>PHMQPFDSGHDDLVHDVVYDFYGRHVATCSSDQHIKVFKLDKDTSNWELSDSWRAHDSSIVAIDWASPEYGRIIASASYDKTVKLWEEDPDQEECSGRRWNKLCTLNDSKGSLYSVKFAPAHLGLKLACLGNDGILRLYDALEPSDLRSWTLTSEMKVLSIPPANHLQSDFCLSWCPSRFSPEKLAVSALEQAIIYQRGKDGKLHVAAKLPGHKSLIRSISWAPSIGRWYQLIATGCKDGRIRIFKITEKLSPLASEESLTNSNMFDNSADVDMDAQGRSDSNTEEKAELQSNLQVELLSEHDDHNGEVWSVSWNLTGTILSSAGDDGKVRLWKATYSNEFKCMSVITAQQ[4x];>MTIDDSNRLLMDVDQFDFLDDGTAQLSNNKTDEEEQLYKRDPVSGAILVPMTVNDQPIEKNGDKMPLKFKLGPLSYQNMAFITAKDKYKLYPVRIPRLDTSKEFSAYVSGLFEIYRDLGDDRVFNVPTIGVVNSNFAKEHNATVNLAMEAILNELEVFIGRVKDQDGRVNRFYELEESLTVLNCLRTMYFILDGQDVEENRSEFIESLLNWINRSDGEPDEEYIEQVFSVKDSTAGKKVFETQYFWKLLNQLVLRGLLSQAIGCIERSDLLPYLSDTCAVSFDAVSDSIELLKQYPKDSSSTFREWKNLVLKLSQAFGSSATDISGELRDYIEDFLLVIGGNQRKILQYSRTWYESFCGFLLYYIPSLELSAEYLQMSLEANVVDITNDWEQPCVDIISGKIHSILPVMESLDSCTAAFTAMICEAKGLIENIFEGEKNSDDYSNEDNEMLEDLFSYRNGMASYMLNSFAFELCSLGDKELWPVAIGL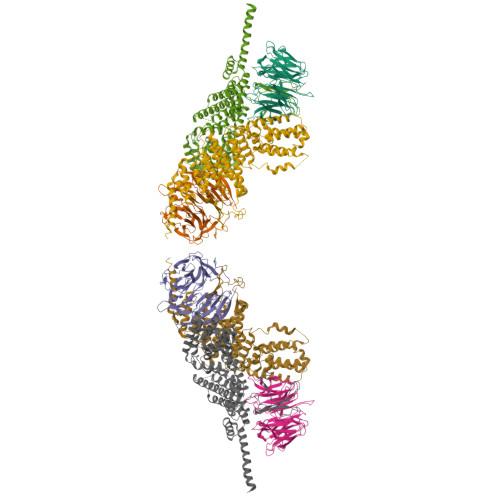IALSATGTRSAKKMVIAELLPHYPFVTNDDIEWMLSICVEWRLPEIAKEIYTTLGNQMLSAHNIIESIANFSRAGKYELVKS[4x]> MAAAAAGAGSGPWAAQEKQFPPALLSFFIYNPRFGPREGQEENKILFYHPNEVEKNEKIRNVGLCEAIVQFTRTFSPSKPAKSLHTQKNRQFFNEPEENFWMVMVVRNPIIEKQSKDGKPVIEYQEEELLDKVYSSVLRQCYSMYKLFNGTFLKAMEDGGVKLLKERLEKFFHRYLQTLHLQSCDLLDIFGGISFFPLDKMTYLKIQSFINRMEESLNIVKYTAFLYNDQLIWSGLEQDDMRILYKYLTTSLFPRHIEPELAGRDSPIRAEMPGNLQHYGRFLTGPLNLNDPDAKCRFPKIFVNTDDTYEELHLIVYKAMSAAVCFMIDASVHPTLDFCRRLDSIVGPQLTVLASDICEQFNINKRMSGSEKEPQFKFIYFNHMNLAEKSTVHMRKTPSVSLTSVHPDLMKILGDI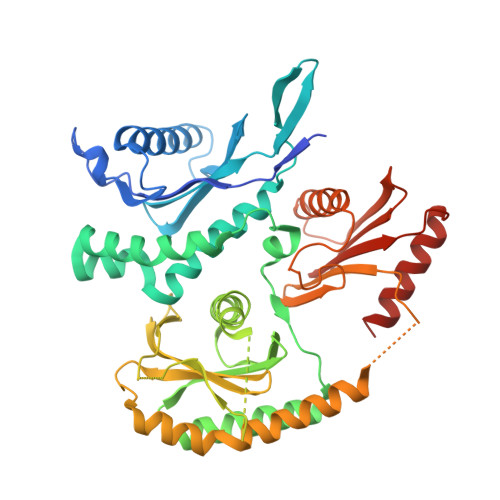NSDFTRVDEDEEIIVKAMSDYWVVGKKSDRRELYVILNQKNANLIEVNEEVKKLCATQFNNIFFLD CT and LT, with their five equivalent binding subunits, are known to be multivalent proteins. Binding has been described as a “two-fingered grip”, provided by the two terminal residues, galactose (Gal) and sialic acid (NeuAc). The specificity of this interaction is mainly determined by the terminal galactose residue, which is buried in a deep pocket at the rugged underside of the toxin (distant from the A-subunit). As expected, all three inhibitors bind in the primary binding site, acting as decoys for the toxins’ main receptor, the GM1 ganglioside.

All three toxins have the same amino acid sequence in the primary binding site, and they have essentially identical 3D structures. pLTB forms crystals under a wider range of conditions than CTB, and the R13H mutation makes the primary binding site identical to that of CTB. The toxin complex with inhibitor 3 was solved to a resolution of 1.6 Å in space group P212121 with one B-pentamer in the asymmetric unit. The inhibitor was present in all five binding sites, and binds in the same manner as 2, with the galactose residue binding to Glu51, Gln61, Asn90 and Lys91, and the sialic acid residue interacting with Glu11 and His13. The benzylamido extension, the feature distinguishing this inhibitor from 2, is flexible and sometimes adopts different conformations. Interestingly, in two of the binding sites, the inhibitor is stretched out and links two adjacent toxin pentamers. In these two cases, the sialic acid moiety extends into the sialic acid binding site of another B-pentamer, creating a cross-over with another ligand. The inhibitor solution was a mixture of two stereoisomers, as indicated by the waved line in Fig. 1. Hence, our data show that the presence of inhibitor 3 shifted the equilibrium towards CTB-dimers (“decamers”). The small increase in oligomerization in solution (20%) measured with SAXS is likely not sufficient to be medically relevant, and the stronger cross-linking effect in cristallo was probably selected for by crystallization.

>APQTITELCSEYHNTQIYTINDKILSYTESMAGKREMVIITFKSGETFQVEVPGSQHIDSQKKAIERMKDTLRITYLTETKIDKLCVWNNKTPNSIAAISMKN[5x]7-(3,5-dimethyl-1~{H}-pyrazol-4-yl)-3-(3-naphthalen-1-yloxypropyl)-1~{H}-indole-2-carboxylic 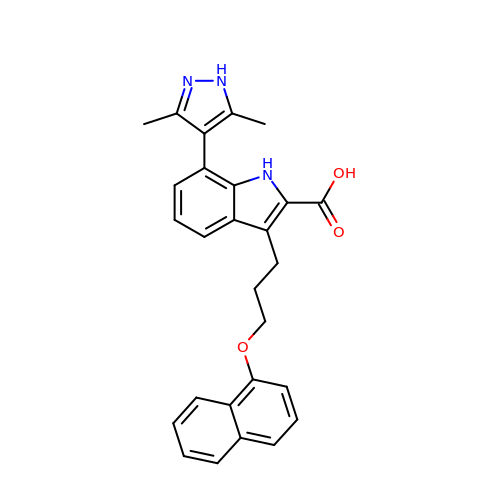acid | C27 H25 N3 O3 | MXUJPYKOCHOAAY-UHFFFAOYSA-N> GPGSEFLTEENFRR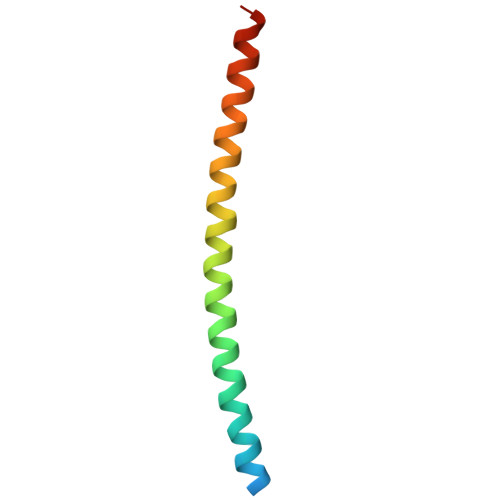LQAEHDRQAKELFLLRKTLEEMELRIETQKQTLNARDESIKKLLEMLQSKGL>YANPVWTALFDYEPSGQDELALRKGDR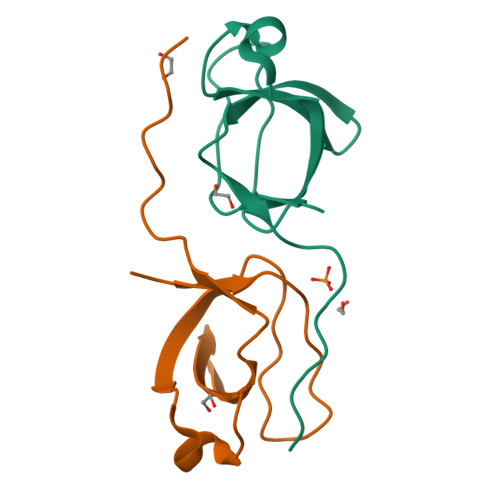VEVLSRDAAISGDEGWWAGQVGGQVGIFPSNYVSRGGGAPPIPPPR[2x]> NQSVVVDFLLPTGVYLNFPVSRNANLSTIKQLLWHRAQYEPLFHMLSGPEAYVFTCINQTAEQQELEDEQRRLCDVQPFLPV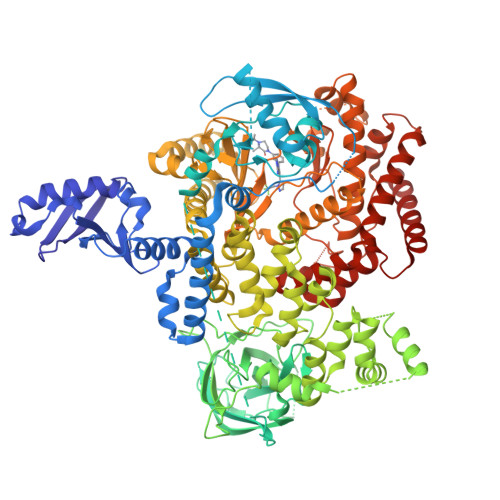LRLVAREGDRVKKLINSQISLLIGKGLHEFDSLCDPEVNDFRAKMCQFCEEAAARRQQLGWEAWLQYSFPLQLEPSAQTWGPGTLRLPNRALLVNVKFEGSEESFTFQVSTKDVPLALMACALRKKATVFRQPLVEQPEDYTLQVNGRHEYLYGSYPLCQFQYICSCLHSGLTPHLTMVHSSSILAMRDEQSNPAPQVQKPRAKPPPIPAKKPSSVSLWSLEQPFRIELIQGSKVNADERMKLVVQAGLFHGNEMLCKTVSSSEVSVCSEPVWKQRLEFDINICDLPRMARLCFALYAVIEKAKKARSTKKKSKKADCPIAWANLMLFDYKDQLKTGERCLYMWPSVPDEKGELLNPTGTVRSNPNTDSAAALLICLPEVAPHPVYYPALEKILELGRHSECVHVTEEEQLQLREILERRGSGELYEHEKDLVWKLRHEVQEHFPEALARLLLVTKWNKHEDVAQMLYLLCSWPELPVLSALELLDFSFPDCHVGSFAIKSLRKLTDDELFQYLLQLVQVLKYESYLDCELTKFLLDRALANRKIGHFLFWHLRSEMHVPSVALRFGLILEAYCRGSTHHMKVLMKQGEALSKLKALNDFVKLSSQKTPKPQTKELMHLCMRQEAYLEALSHLQSPLDPSTLLAEVCVEQCTFMDSKMKPLWIMYSNEEAGSGGSVGIIFKNGDDLRQDMLTLQMIQLMDVLWKQEGLDLRMTPYGCLPTGDRTGLIEVVLRSDTIANIQLNKSNMAATAAFNKDALLNWLKSKNPGEALDRAIEEFTLSCAGYCVATYVLGIGDRHSDNIMIRESGQLFHIDFGHFLGNFKTKFGINRERVPFILTYDFVHVIQQGKTNNSEKFERFRGYCERAYTILRRHGLLFLHLFALMRAAGLPELSCSKDIQYLKDSLALGKTEEEALKHFRVKFNEALRESWKT;> YQQDQVVKEDNIEAVGKKLHEYNTQFQEKSREYDRLYEDYTRTSQEIQMKRTAIEAFNETIKIFEEQCQTQERYSKEYIEKFKREGNETEIQRIMHNYEKLKSRISEIVDSRRRLEEDLKKQAAEYREIDKRMNSIKPDLIQLRKTRDQYLMWLTQKGVRQKKLNEWLGN> GSVTFEFENLSEEAAEKVKKYVKEVAEKLGVEVKVEEEEGKLKIYVENLKEEDALDIFK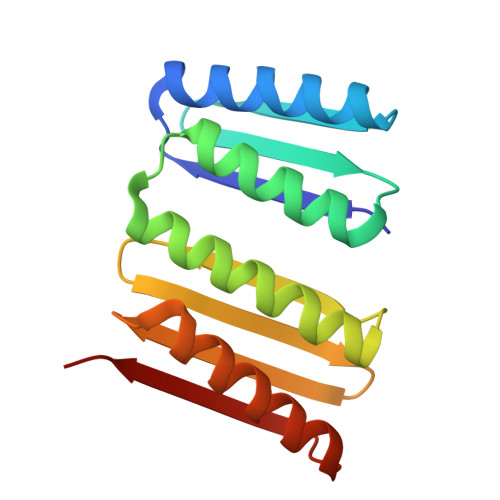YAALAAELDQEYLDMVEAAIKAYHLFKEYDENATIEITIDDEGIEVKVESGDRVVTLKFKNVSKEEVEEAVKEALKQLEAGQKKVEVEVEGGS> MIAEELLRAGRLDDALKALQEQVRSQPSNATLRIFLFQLLAVMGQWARAQNQLKVVGELDASALPMVQTYSTAIDCEALRREVFAGRLTPVILGQPAEWIAPLLQALSLDAEGHGEAAQALREQAFDAAPAVPGRIGEAPFAWLADA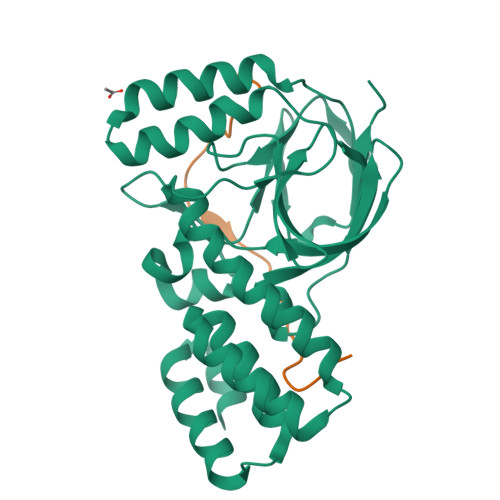DTRLGPVLEVIVNGRYAWLPMSNLRSLKVEAPSDLRDLVWLPAELTLANGGATVALLPARYAETVEHGDDAARLGRKTEWLDSGLPVGQRLFVTDAGETALFDLRELDFEPTDA;> MGSTTSSQKFIARNRAPRVQIEYDVELYGAEKKVQLPFVMGVMADLAGKPAEPQAAVADRKFLEIDVDNFDARLKAMKPRVAFNVPNVLTGEGNLSLDITFESMDDFSPAAVARKVDSLNKLLEARTQLANLLTYMDGKTGAEEMIMKAIKDPALLQALASAPKPKDDEPQA>[2x]MHHHHHHSSGRENLYFQGVDLELRVLEESDLSSHLELLGHLTEAPPLSGVELANIADMRRRAGIVTKVFCHQPTGRIVGSASLMIQPKFTRGGRAVGHIEDVVVDPSYRGAGLG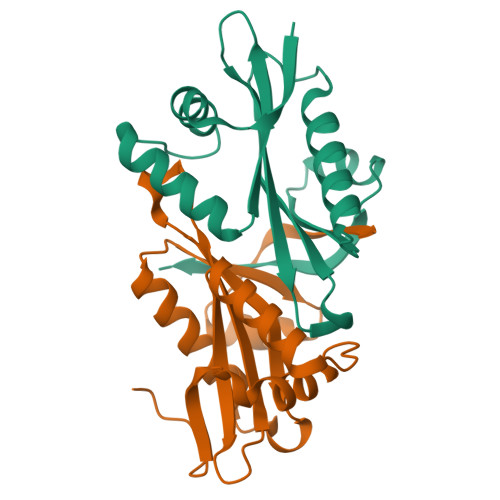KALIMDLCEISRSKGCYKVILDSSEKSLPFYEKLGFRAHERQMRLDL> AUGCGCCCAGAUAGGGUGUUAAGUCAAGUAGUUUAAGGUACUACUCUGUAAGAUAACACAGAAAACAGCCAACCUAACCGAAAAGCGAAAGCUGAUACGGGAACAGAGCACGGUUGGAAAGCGAUGAGUUACCUAAAGACAAUCGGGUACGACUGAGUCGCAAUGUUAAUCAGAUAUAAGGUAUAAGUUGUGUUUACUGAACGCAAGUUUCUAAUUUCGGUUAUGUGUCGAUAGAGGAAAGUGUCUGAAACCUCUAGUACAAAGAAAGGUAAGUUAUGGUUGUGGACUUAUCUGUUAUCACCACAUUUGUACAAUCUGUAGGAGAACCUAUGGGAACGAAACGAAAGCGAUGCCGAGAAUCUGAAUUUACCAAGACUUAACACUAACUGGGGAUACCCUAAACAAGAAUGCCUAAAGGAGGAAAAAGGCUAUAGCACUAGAGCUUGAAAAUCUUGCAAGGGUACGGAGUACUCGUAGUA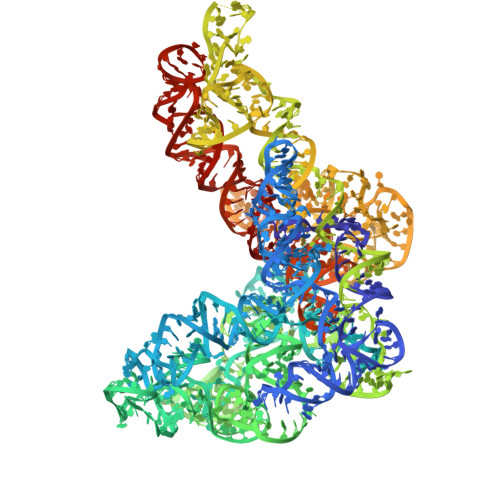GUCUGAGAAGGGUAACGCCCUUUACAUGGCAAAGGGGUACAGUUAUUGUGUACUAAAAUUAAAAAUUGAUUAGGGAGGAAAACCUCAAACCAACAAUGGCAAUUUUAGACAAUAACAGAGCCGUAUACUCCGAGAGGGGUACGUACGGUUCCCGAAGAGGGUGGUGCAAACCAGUCACAGUAAUGUGAACAAGGCGGUACCUCCCUACUUCACCACAUCCAUAAC> MRGSHHHHHHGSALSNKFIGDDMKMTYHMDGCVNGHYFTVKGEGNGKPYEGTQTSTFKVTMANGGPLAFSFDI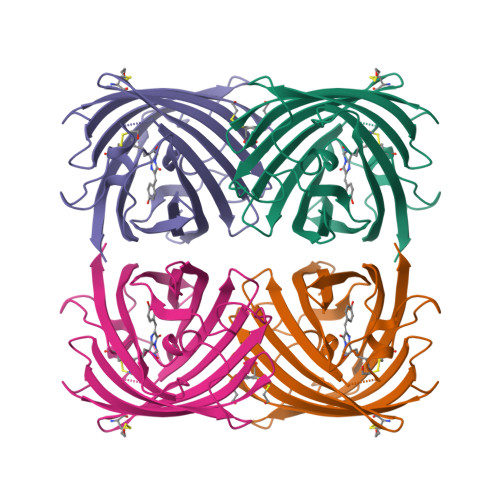LSTVFKYGNRCFTAYPTSMPDYFKQAFPDGMSYERTFTYEDGGVATASWEISLKGNCFEHKSTFHGVNFPADGPVMAKKTTGWDPSFQKMTVCDGILKGDVTAFLMLQGGGNYRCQFHTSYKTKKPVTMPPNHVVEHRIARTDLDKGGNSVQLTEHAVAHITSVVPF> MASSRCPAPRGCRCLPGASLAWLGTVLLLLADWVLLRTALPRIFSLLVPTALPLLRVWAVGLSRWAVLWLGACGVLRATVGSKSENAGAQGWLAALKPLAAALGLALPGLALFRELISWGAPGSADSTRLLHWGSHPTAFVVSYAAALPAAALWHKLGSLWVPGGQGGSGNPVRRLLGCLGSETRRLSLFLVLVVLSSLGEMAIPFFTGRLTDW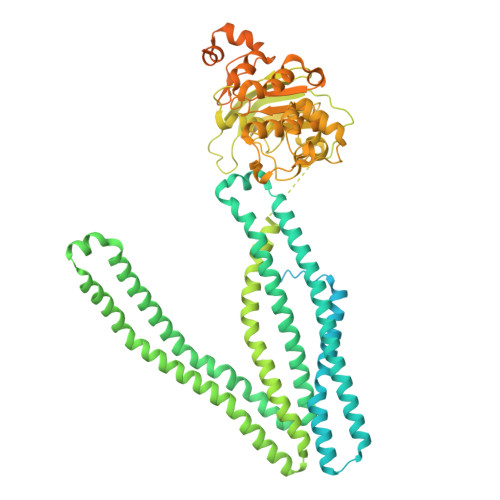ILQDGSADTFTRNLTLMSILTIASAVLEFVGDGIYNNTMGHVHSHLQGEVFGAVLRQETEFFQQNQTGNIMSRVTEDTSTLSDSLSENLSLFLWYLVRGLCLLGIMLWGSVSLTMVTLITLPLLFLLPKKVGKWYQLLEVQVRESLAKSSQVAIEALSAMPTVRSFANEEGEAQKFREKLQEIKTLNQKEAVAYAVNSWTTSISGMLLKVGILYIGGQLVTSGAVSSGNLVTFVLYQMQFTQAVEVLLSIYPRVQKAVGSSEKIFEYLDRTPRCPPSGLLTPLHLEGLVQFQDVSFAYPNRPDVLVLQGLTFTLRPGEVTALVGPNGSGKSTVAALLQNLYQPTGGQLLLDGKPLPQYEHRYLHRQVAAVGQEPQVFGRSLQENIAYGLTQKPTMEEITAAAVKSGAHSFISGLPQGYDTEVDEAGSQLSGGQRQAVALARALIRKPCVLILDDATSALDANSQLQVEQLLYESPERYSRSVLLITQHLSLVEQADHILFLEGGAIREGGTHQQLMEKKGCYWAMVQAPADAPESAQLEGSGGGAMVTTLSGLSGEQGPSGDMTTEEDSATHIKFSKRDEDGRELAGATMELRDSSGKTISTWISDGHVKDFYLYPGKYTFVETAAPDGYEVATPIEFTVNEDGQVTVDGEATEGDAHTSGGGHHHHHHHHHH> MVPISPIETVPVKLKPGMDGPKVKQWPLTEEKIKALVEICTEMEKEGKISKIGPENPYNTPVFAIKKKDSTKWRKLVDFRELNKRTQDFWEVQLGIPHPAGLKKKKSVTVLDVGDAYFSVPLDEDFRKYTAFTIPSINNETPGIRYQYNVLPQGWKGSPAIFQSSMTKILEPFKKQNPDIVIYQYMDDLYVGSDLEIGQHRTKIEELRQHLLRWGLTTPD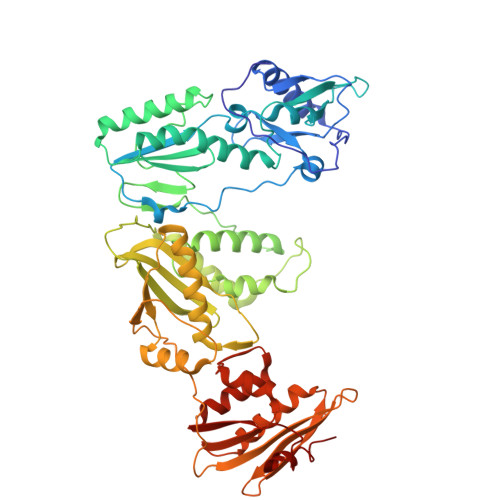KKHQKEPPFLWMGYELHPDKWTVQPIVLPEKDSWTVNDICKLVGKLNWASQIYPGIKVRQLSKLLRGTKALTEVIPLTEEAELELAENREILKEPVHGVYYDPSKDLIAEIQKQGQGQWTYQIYQEPFKNLKTGKYARMRGAHTNDVKQLTEAVQKITTESIVIWGKTPKFKLPIQKETWETWWTEYWQATWIPEWEFVNTPPLVKLWYQLEKEPIVGAETFYVDGAANRETKLGKAGYVTNKGRQKVVPLTNTTNQKTELQAIYLALQDSGLEVNIVTNSQYALGIIQAQPDKSESELVNQIIEQLIKKEKVYLAWVPAHKGIGGNEQVDKLVSA> MANYWLYKSEPFKWSWEMQKAKGETGEEWTGVRNYQARNNMRAMKIGDKGFFYHSNEGLDVVGIVEV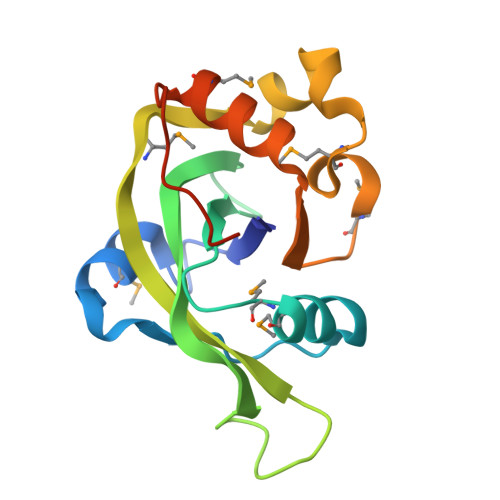CALSHPDSTAEGDLKWDCVDIRAVCDMPQPVSLKDVKANPKLEKMSLVTSMRLSVQPVTEEEYLEVCRMGGLANPPKSPDLEHHHHHH PgDPP11 exhibits a strict substrate specificity for acidic residues (Asp/Glu) at the P1 position (NH2-P2-P1-P1’-P2’-…, where the P1-P1’ bond is the scissile bond), whereas PgDPP7 exhibits a broad substrate specificity for both aliphatic and aromatic residues at the P1 position. PgDPP11 is a homodimer, and each subunit contains a peptidase domain, including a double β-barrel fold that is characteristic of the chymotrypsin superfamily, as well as an unusual α-helical domain that regulates the exopeptidase activity of PgDPP11. Biochemical studies and crystal structure analyses revealed that Arg673 in the S1 subsite of PgDPP11 is a crucial residue for the strict Asp/Glu P1 specificity of PgDPP1123,27,31.

The screening resulted in the first nonpeptidyl inhibitor of S46 peptidases, SH-5 (2-[(2-aminoethyl)amino]-5-nitrobenzoic acid, C9H11N3O4). The binding mode of SH-5 was confirmed by crystal structure analysis at a 2.39 Å resolution. The crystal structure of PgDPP11 complexed with SH-5 (yellow) showed that the carboxy group of SH-5 forms an electrostatic interaction with the side chain of Arg673, a crucial residue for the Asp/Glu specificity of PgDPP1123,27,31. This experimental observation is consistent with the previously obtained in silico docking model based on MM-GBSA scoring (light green). The crystal structure of the SH-5 complex also revealed that the 5-nitro group of SH-5 is involved in a hydrogen bond network with the side chains of Thr650 and Asn670. An amino acid sequence comparison of residues in the S1 subsite of typical S46 peptidases shows that Thr650 and Asn670 in PgDPP11 are well conserved among DPP11s but are replaced by hydrophobic residues, namely, Ile and Ala, respectively, in DPP7s. This result indicates that the hydrogen bond network between Thr650 and Asn670 exists specifically in DPP11s (but not in DPP7s), and the nitro group of SH-5 (and its analog) is also important for the selectivity of this type of inhibitor against DPP11s over DPP7s. For the selectivity, the electrostatic interaction between Arg673 and the carboxy group of SH-5 appears to be more dominant than the hydrogen bond network involving Thr650, Asn670 and the nitro group of SH-5, because Arg673 is replaced by Ser667 in SmDPP11. The Ki vales of SH-5 and the lipophilic analog NPPB against PgDPP11 were estimated to be 8.45 and 15.0 μM, respectively. The target selectivity of the inhibitor, that is the inhibitory effects against DPP11s over DPP7s, is explained by a specific hydrogen bond network and an electrostatic interaction between the inhibitor and the active site residues of PgDPP11 that are conserved among DPP11s but not in DPP7s.

>MKKRLLLPLFAALCLSQIAHADEGMWLMQQLGRKYAQMKERGLKMKEYDLYNPNGTSLKDAVVLFDGGCTGEVVSDRGLVLTNHHCGYDMIQAHSTLEHNYLENGFWAMREADELPNKDISVVFIDKIEDVTDYVKKELKAIKDPNSMDYLSPKYLQKLADKKAGKNFSAKNPGLSVEIKAFYGGNLYLMFTKKTYTDVRLVGAPPSSIGKFGADTDNWIWPRHTGDFSIFRIYADKNGNPAPYSEDNVPLKPKRFFNISLGGVQENDYAMIMGFPGTTHRYFTASEVDEWKSIDNDIRIRMRDIRQGVMLREMLADPQIKIMYSAKYAASQNAYKRAIGANWAIKTRGLRQNKQAMQDRLIAWGAKQGTPRYEEAVHEIDATVAKRADLRRRYWMIEEGIIRGIEFARSPIPTEDETKALQGNDASARKEAIDKIRTRYSKFANKDYSAEVDKKVAVAMLTEYLKEIPYENLPLHLRLVKDRFAGDVQAYVDDIFARSVFGSEAQFDAFAAVPSVEKLAEDPMVLFASSVFDEYRKLYNELRPYDDPILRAQRTYIAGLLEMDGDQDQFPDANLTLRFTYGQVKGYSPRDNVYYGHQTTLDGVMEKEDPDNWEFVVDPKLKAVYERKDFGRYADRSGRMPVAFCATTHTTGGNSGSPVMNANGELIGLNFDRNWEGVGGDIQYLADYQRSIIVDIRYVLLVIDKVGGCQRLLDEMNIVP[2x]>MARDHRKIGRDQELYFFHELSPGSCFFLPKGAYIYNALIEFIRSEYRKRGFQEVVTPNIFNSRLWMTSGHWQHYSENMFSFEVEKELFALKPMNCPGHCLMFDHRPRSWRELPLRLADFGVLHRNELSGALTGLTRVRRFQQDDAHIFCAMEQIEDEIKGCLDFLRTVYSVFGFSFKLNLSTRPEKFLGDIEVWDQAEKQLENSLNEFGEKWELNSGDGAFYGPKIDIQIKDAIGRYHQCATIQLDFQLPIRFNLTYVSHDGDDKKRPVIVHRAILGSVERMIAILTENYGGKWPFWLSPRQVMVVPVGPTCDEYAQKVRQQFHDAKFMADIDLDPGCTLNKKIRNAQLAQYNFILVVGEKEKISGTVNIRTRDNK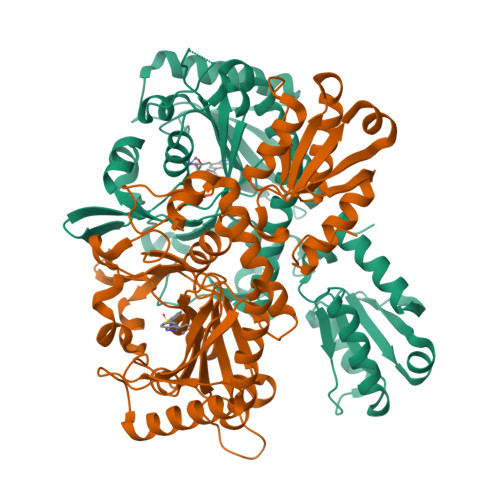VHGERTISETIERLQQLKEFRSKQAEEEFLEHHHHHH[2x]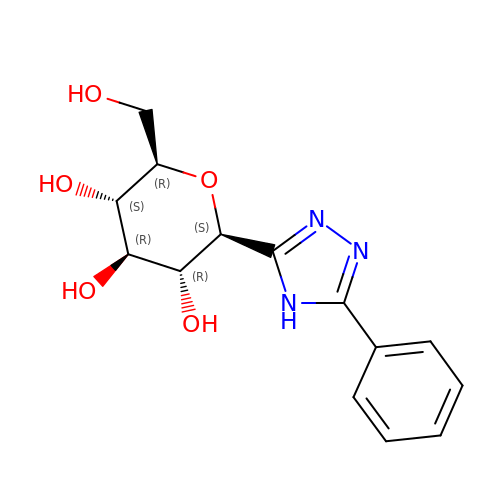(1S)-1,5-anhydro-1-[3-(4-hydroxyphenyl)-1H-1,2,4-triazol-5-yl]-D-glucitol | C14 H17 N3 O5 | GTQQOMHOHKJYAX-RMPHRYRLSA-N>GPKEWQENKSWNAHFTEHKSQGVVVLWNENKQQGFTNNLKRANQAFLPASTFKIPNSLIALDLGVVKDEHQVFKWDGQTRDIATWNRDHNLITAMKYSVVPVYQEFARQIGEARMSKMLHAFDYGNEDISGNVDSFWLDGGIRISATEQISFLRKLYHNKLHVSERSQRIVKQAMLTEANGDYIIRAKTGYSPKIGWWVGWVELDDNVWFFAMNMDMPTSDGLGLRQAITKEVLKQEKIIP[2x]

The OXA-48 carbapenemase is widely disseminated in Enterobacterales, necessitating new treatments for producer strains. OXA-48 is a class D SBL that uses a nucleophilic serine (Ser70) to hydrolyse β-lactams, with a proximal post-translationally carbamylated lysine (Lys73) proposed to act as the general base for both the acylation and deacylation steps of the reaction. Diazabicyclooctane (DBO) inhibitors, including avibactam and nacubactam, act on a wide range of enzymes to overcome β-lactamase-mediated resistance. Here we describe investigations on how avibactam and nacubactam inhibit OXA-48 and two variants, OXA-163 and OXA-405, with deletions in the β5–β6 loop neighbouring the active site that modify activity towards different β-lactam classes.

Nacubactam is distinguished from avibactam by an extended C2 substituent bearing a 1-aminoethoxy group. Both OXA-163 and OXA-405 have four amino acid deletions within the β5–β6 loop, including of residue Arg214. In the carbamoyl-enzyme complexes with OXA-405 and OXA-163, both nacubactam and avibactam adopt similar binding modes to those observed with OXA-48. These are characterised by complementary electrostatic interactions between the DBO sulfate group and Arg250 (OXA-48 numbering) and positioning of their C2 tail groups close to the β5–β6 loop. The C2 substituent of avibactam is identically positioned in all three enzyme complexes, whereas the additional 1-aminoethoxy group of nacubactam appears more variably located across these structures. Lys73 is fully decarbamylated in all DBO-bound structures except the OXA-405 : avibactam (both chains), OXA-163 : avibactam (only in chain A) and 16 hour OXA-163 : nacubactam (both chains) complexes, where Lys73 is modelled as partially carbamylated, in dual-occupancy with a free lysine side-chain that is associated with either a water molecule or chloride ion. Leu158 appears to adopt an alternative rotamer (g−) when avibactam is bound to OXA-163 (chain B) and OXA-405 (both chains), compared to OXA-48 or chain A of the OXA-163 : avibactam complex where the t-rotamer is observed. A hydroxylamine desulfated carbamoyl-enzyme was also modelled in dual occupancy with the intact avibactam- and nacubactam-derived complexes of both OXA-163 and OXA-405. We also see evidence of desulfation in our crystal structures of OXA-163 and OXA-405 bound to both avibactam and nacubactam, indicated by negative Fo–Fc difference density around the DBO sulfate group when only the intact carbamoyl-enzyme is modelled. The desulfated hydroxylamine group can form hydrogen bond networks with the active sites of OXA-163 and OXA-405 via a water molecule, observed in a similar position to an equivalent water in structures of the uncomplexed enzymes, that is in dual occupancy with the intact carbamoyl-enzyme sulfate group.N-[2-({N-[(2R)-2-hydroxy-3,3-dimethyl-4-(phosphonooxy)butanoyl]-beta-alanyl}amino)ethyl]-L-leucinamide | C17 H35 N4 O8 P | 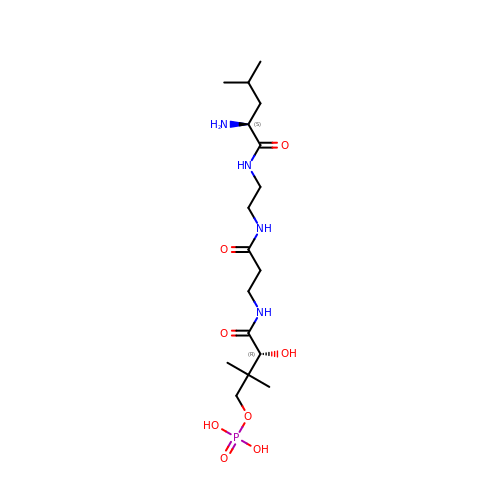OHVFVHYHCFDMRA-JSGCOSHPSA-N> MTMDATALPSELLVTPQPLVGFCGLDTARVSVHKAVWEAFSGSLQRKAADRAAVQYKLLPPNYEFPVAKPKRASYEWYHPKGILKRNWMLKHLHVLPSVVVLFQDMEWNDLQWTEKQVQCAAIVQALKNTLQERNTRLCLVLLQRAAPLPPGEDLLAAERAASLTNACGITSKMLFILPHTEHLTGYALRLESAFLDMAQS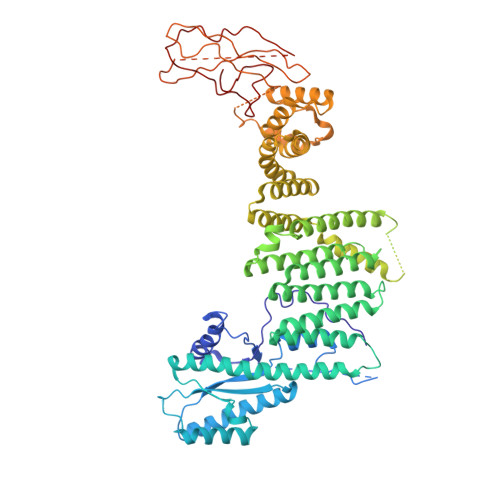YYALMSKRIRNHRDQLTAAHTSLKIRHQFKLGFVAEMRQDFSTGQKHYFQAYANLDEIRINDGNCLEIKTLAGFLNYKICRLMFKLKTPRDAINQFIIHVEKHKSRVGFKDLAFEHHAWLSTQHSVFAELFCEAIKNGLPALQTQHPGIYYHKAAEFVMKRRDAAMEAYAAMQASSEATPTPIQNPLSLYTEFFGIRAVKTGDLVAEQQANMQLCDQERSYNHSAAIIALLSQAMAQFKIYKCLRFRKKLAIDMAEEYLKSGDHAKALTLYSLMLPDYRQEKWTTIFTDVLLKTLRCALLSGSVADYIACSVEALSLRHQSDQSERILILENLWQVFQGVPPMPKTQLTPEAQALWTSALANVKSPIQIDLDKVNDVVEMCATFERVQLSNDDLLQLQLIVRVLTDIPLRIRSFHVILADAGNPQNSYKLEALKYFCFPTLTQLRGQKQPDDEQLENPSQEPKNFEKNMRLEPGSYYQLFCSTEAQQFHENTQLRIVRLEAHMGTDQVAALLTCSSN> GAMEATEIISTLSNGLIASHYGVSFFTIQSFVSSLSNTSTLKNMLYVLSTAVEFESVPLRKGDRALLVKLSKRLPLRFPEHTSSGSVSFKVFLLLQAYFSRLELPVDFQNDLKDILEKVVPLINVVVDILSANGYLNATTAMDLAQMLIQGVWDVDNPLRQIPHFNNKILEKCKEINVETVYDIMALEDEERDEILTLTDSQLAQVAAFVNNYPNVELTYSLNNSDSLISGVKQKITIQLTRDVEPENLQVTSEKYPFDKLESWWLVLGEVSKKELYAIKKVTLNKETQQYELEFDTPTSGKHNLTIWCVCDSYLDADKEL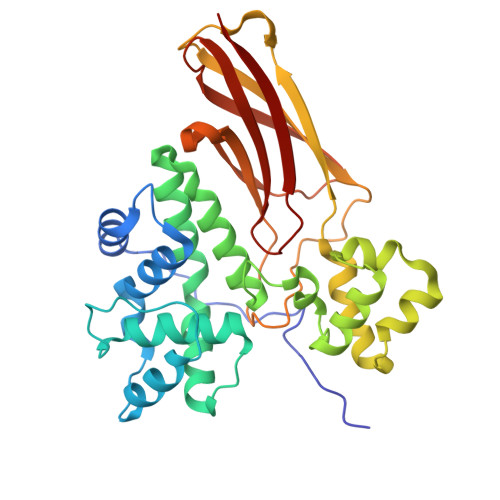SFEINVK>[3x]GHMPLLSASIVSAPVVTSETYVDIPGLYLDVAKAGIRDGKLQVILNVPTPYATGNNFPGIYFAIATNQGVVADGCFTYSSKVPESTGRMPFTLVATIDVGSGVTFVKGQWKSVRGSAMHIDSYASLSAIWGTAA

BC2L-C also presented at its N-terminus a domain of unknown function, which was later revealed to be also a lectin domain (BC2L-CN). Establishing a new lectin family, BC2L-CN showed specificity for fucosides, especially blood group antigens, for which the measured affinity reached micromolar range. BC2L-CN was the first lectin to display a trimeric arrangement of the jelly roll fold primarily observed in tumor necrosis factor α (TNF-α). A novel binding site and binding mode for fucosides was also uncovered at each interface between two protomers, which implicated an essential arginine residue.

We also determined the thermodynamic parameters for the interaction of rBC2L-CN2 with Globo H. This hexasaccharide contains the H-type 3 antigen (Fucα1-2Galβ1-3GalNAc), previously shown to be recognized by BC2L-CN in cell binding assays and in glycan arrays. We measured a Kd of 26 µM, which classified Globo H as the best ligand to date for BC2L-CN. The structure of the H-type 1 complex belongs to space group R32:h (H32, a = b = 42.7 Å, c = 308.6 Å) with one monomer in the asymmetric unit, whereas the one of the H-type 3 complex belongs to the C2 space group (a = 74.4 Å, b = 42.9 Å, c = 102.6 Å and β = 96.0°) with one trimer in the asymmetric unit. For the structure in complex with Globo H hexasaccharide, the four units were modelled in every protein chain and the fifth one only in protein chains B and C. No electron density was visible for the reducing glucose, which, likewise, was completely solvent exposed. The following N-acetylated sugar, GlcNAc in H-type 1 or GalNAc in H-type 3, interacted mainly with its acetyl group. In some chains, the acetyl group’s oxygen also established a hydrogen bond mediated by a water molecule with both the next glycosidic oxygen and the main chain of Thr83. For the remaining sugar units in the Globo H structure, most of the interactions were seen in protein chain C and are depicted in Figure 3F. The O6 and O4 hydroxyls of the fourth sugar (Gal4) made a water-mediated hydrogen bond with the main chain oxygen of Glu81. In the α1-4 linked galactose (Gal5), only one interaction was observed between the O6 and the side chain of Lys78 from the neighboring chain. Those interactions with Gal4 and Gal5 were not seen in the protein chain B as a result of a different orientation of the O6 of Gal4 and of the terminal nitrogen of Lys78. In protein chain A no density was visible after Gal4, which presented different torsion angles than in the other chains, resulting in a more solvent-exposed sugar.> GP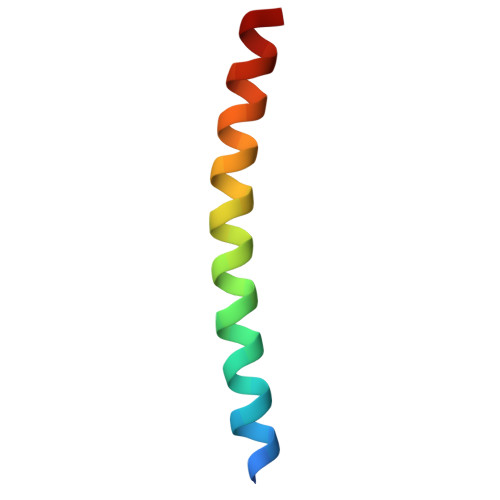LGSNRRLQQTQAQVDEVVDIMRVNVDKVLERDQKL> X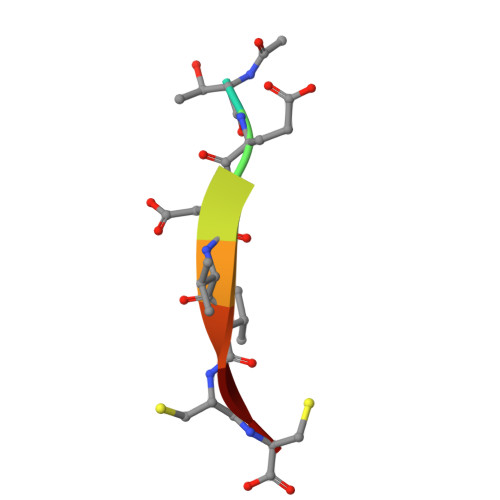TEDVVCC> GHAADRIARLPGQPAVDFDMYSGYITVDEGAGRSLFYLLQEAPEDAQPAPLVLWLNGGPGCSSVAYGASE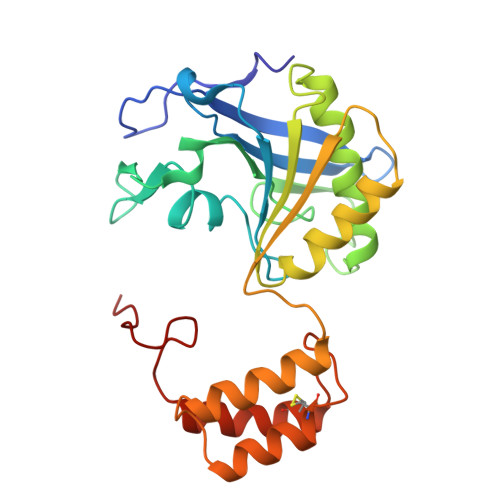ELGAFRVKPRGAGLVLNEYRWNKVANVLFLDSPAGVGFSYTNTSSDIYTSGDNRTAHDSYAFLAKWFERFPHYKYRDFYIAGESYAGHYVPELSQLVHRSKNPVINLKGFMVGNGLIDDYHDYVGTFEFWWNHGIVSDDTYRRLKEACLHDSFIHPSPACDAATDVATAEQGNIDMYSLYTPVCNI>MEPHVLGAVLYWLLLPCALLAACLLRFSGLSLVYLLFLLLLPWFPGPTRCGLQGHTGRLLRALLGLSLLFLVAHLALQICLHIVPRLDQLLGPSCSRWETLSRHIGVTRLDLKDIPNAIRLVAPDLGILVVSSVCLGICGRLARNTRQSPHPRELDDDERDVDASPTAGLQEAATLAPTRRSRLAARFRVTAHWLLVAAGRVLAVTLLALAGIAHPSALSSVYLLLFLALCTWWACHFPISTRGFSRLCVAVGCFGAGHLICLYCYQMPLAQALLPPAGIWARVLGLKDFVGPTNCSSPHALVLNTGLDWPVYASPGVLLLLCYATASLRKLRAYRPSGQRKEAAKGYEARELELAELDQWPQERESDQHVVPTAPDTEADNCIVHELTGQSSVLRRPVRPKRAEPREASPLHSLGHLIMDQSYVCALIAMMVWSITYHSWLTFVLLLWACLIWTVRSRHQLAMLCSPCILLYGMTLCCLRYVWAMDLRPELPTTLGPVSLRQLGLEHTRYPCLDLGAMLLYTLTFWLLLRQFVKEKLLKWAESPAALTEVTVADTEPTRTQTLLQSLGELVKGVYAKYWIYVCAGMFIVVSFAGRLVVYKIVYMFLFLLCLTLFQVYYSLWRKLLKAFWWLVVAYTMLVLIAVYTFQFQDFPAYWRNLTGFTDEQLGDLGLEQFSVSELFSSILVPGFFLLACILQLHYFHRPFMQLTDMEHVSLPGTRLPRWAHRQDAVSGTPLLREEQQEHQQQQQEEEEEEEDSRDEGLGVATPHQATQVPEGAAKWGLVAERLLELAAGFSDVLSRVQVFLRRLLELHVFKLVALYTVWVALKEVSVMNLLLVVLWAFALPYPRFRPMASCLSTVWTCVIIVCKMLYQLKVVNPQEYSSNCTEPFPNSTNLLPTEISQSLLYRGPVDPANWFGVRKGFPNLGYIQNHLQVLLLLVFEAIVYRRQEHYRRQHQLAPLPAQAVFASGTRQQLDQDLLGCLKYFINFFFYKFGLEICFLMAVNVIGQRMNFLVTLHGCWLVAILTRRHRQAIARLWPNYCLFLALFLLYQYLLCLGMPPALCIDYPWRWSRAVPMNSALIKWLYLPDFFRAPNSTNLISDFLLLLCASQQWQVFSAERTEEWQRMAGVNTDRLEPLRGEPNPVPNFIHCRSYLDMLKVAVFRYLFWLVLVVVFVTGATRISIFGLGYLLACFYLLLFGTALLQRDTRARLVLWDCLILYNVTVIISKNMLSLLACVFVEQMQTGFCWVIQLFSLVCTVKGYYDPKEMMDRDQDCLLPVEEAGIIWDSVCFFFLLLQRRVFLSHYYLHVRADLQATALLASRGFALYNA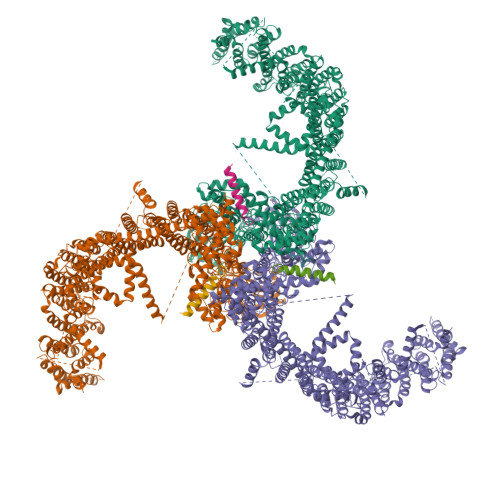ANLKSIDFHRRIEEKSLAQLKRQMERIRAKQEKHRQGRVDRSRPQDTLGPKDPGLEPGPDSPGGSSPPRRQWWRPWLDHATVIHSGDYFLFESDSEEEEEAVPEDPRPSAQSAFQLAYQAWVTNAQAVLRRRQQEQEQARQEQAGQLPTGGGPSQEVEPAEGPEEAAAGRSHVVQRVLSTAQFLWMLGQALVDELTRWLQEFTRHHGTMSDVLRAERYLLTQELLQGGEVHRGVLDQLYTSQAEATLPGPTEAPNAPSTVSSGLGAEEPLSSMTDDMGSPLSTGYHTRSGSEEAVTDPGEREAGASLYQGLMRTASELLLDRRLRIPELEEAELFAEGQGRALRLLRAVYQCVAAHSELLCYFIIILNHMVTASAGSLVLPVLVFLWAMLSIPRPSKRFWMTAIVFTEIAVVVKYLFQFGFFPWNSHVVLRRYENKPYFPPRILGLEKTDGYIKYDLVQLMALFFHRSQLLCYGLWDHEEDSPSKEHDKSGEEEQGAEEGPGVPAATTEDHIQVEARVGPTDGTPEPQVELRPRDTRRISLRFRRRKKEGPARKGAAAIEAEDREEEEGEEEKEAPTGREKRPSRSGGRVRAAGRRLQGFCLSLAQGTYRPLRRFFHDILHTKYRAATDVYALMFLADVVDFIIIIFGFWAFGKHSAATDITSSLSDDQVPEAFLVMLLIQFSTMVVDRALYLRKTVLGKLAFQVALVLAIHLWMFFILPAVTERMFNQNVVAQLWYFVKCIYFALSAYQIRCGYPTRILGNFLTKKYNHLNLFLFQGFRLVPFLVELRAVMDWVWTDTTLSLSSWMCVEDIYANIFIIKCSRETEKKYPQPKGQKKKKIVKYGMGGLIILFLIAIIWFPLLFMSLVRSVVGVVNQPIDVTVTLKLGGYEPLFTMSAQQPSIIPFTAQAYEELSRQFDPQPLAMQFISQYSPEDIVTAQIEGSSGALWRISPPSRAQMKRELYNGTADITLRFTWNFQRDLAKGGTVEYANEKHMLALAPNSTARRQLASLLEGTSDQSVVIPNLFPKYIRAPNGPEANPVKQLQPNEEADYLGVRIQLRREQGAGATGFLEWWVIELQECRTDCNLLPMVIFSDKVSPPSLGFLAGYGIMGLYVSIVLVIGKFVHGFFSEISHSIMFEELPCVDRILKLCQDIFLVRETRELELEEELYAKLIFLYRSPETMIKWTREKE[3x];>MSGAGEALAPGPVGPQRVAEAGGGQLGSTAQGKCDKDNTEKDITQATNSHFTHGEMQDQSIWGNPSDGELIRTQPQRLPQLQTSAQVPSGEEIGKIKNGHTGLSNGNGIHHGAKHGSADNRKLSAPVSQKMHRKIQSSLSVNSDISKKSKVNAVFSQKTGSSPEDCCVHCILACLFCEFLTLCNIVLGQASCGICTSEACCCCCGDEMGDDCNCPCDMDCGIMDACCESSDCLEICMECCGICFPS[3x]> SQNLTCNSNDLKALEGFMRGLESSIDGWKWNESSSFSSNCCDWVGISCKSSVSLGLDDVNESGRVVELELGRRKLSGKLSESVAKLDQLKVLNLTHNSLSGSIAASLLNLSNLEVLDLSSNDFSGLFPSLINLPSLRVLNVYENSFHGLIPASLCNNLPRIREIDLAMNYFDGSIPVGIGNCSSVEYLGLASNNLSGSIPQELFQLSNLSVLALQNNRLSGALSSKLGKLSNLGRLDISSNKFSG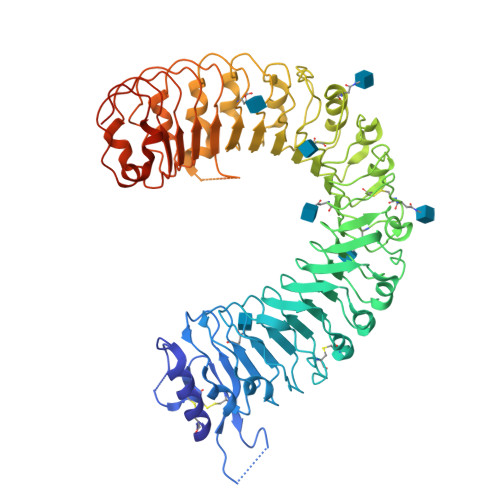KIPDVFLELNKLWYFSAQSNLFNGEMPRSLSNSRSISLLSLRNNTLSGQIYLNCSAMTNLTSLDLASNSFSGSIPSNLPNCLRLKTINFAKIKFIAQIPESFKNFQSLTSLSFSNSSIQNISSALEILQHCQNLKTLVLTLNFQKEELPSVPSLQFKNLKVLIIASCQLRGTVPQWLSNSPSLQLLDLSWNQLSGTIPPWLGSLNSLFYLDLSNNTFIGEIPHSLTSLQSLVSKENAVEEPSPDFPFFKKKNTNAGGLQYNQPSSFPPMIDLSYNSLNGSIWPEFGDLRQLHVLNLKNNNLSGNIPANLSGMTSLEVLDLSHNNLSGNIPPSLVKLSFLSTFSVAYNKLSGPIPTGVQFQTFPNSSFEGNQGLCGEHASPCHITDQSPHGSHHHHHH> MSGLDKYLPGIEKLRRGDGEVEVKSLAGKLVFFYFSAS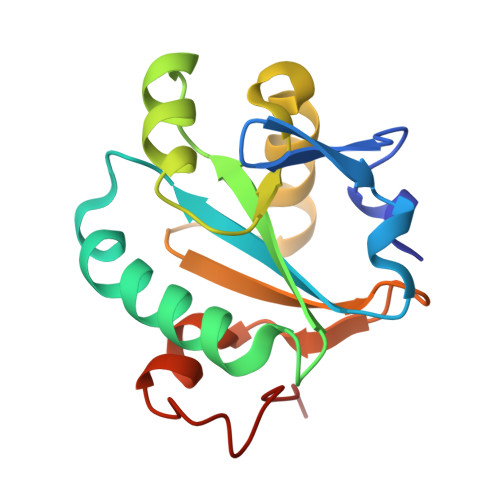WCPPARGFTPQLIEFYDKFHESKNFEVVFCTWDEEEDGFAGYFAKMPWLAVPFAQSEAVQKLSKHFNVESIPTLIGVDADSGDVVTTRARATLVKDPEGEQFPWKDAP> MGNDDIRQVYYEDKGISHAKAGRYSQAVMLLEQVYDADAFDVDVALHLGIAYVKTGAVDRGTELLERSLADAPDNVKVATVLGLTYVQVQKYDLAVPLLIKVAEANPINFNVR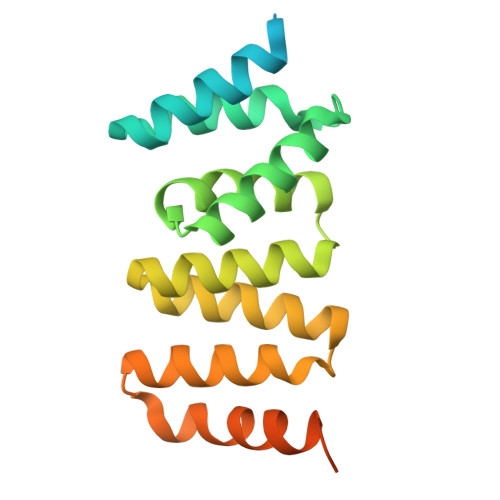FRLGVALDNLGRFDEAIDSFKIALGLRPNEGKVHRAIAFSYEQMGRHEEALPHFKKANELDEGASVELALVPRGSSAHHHHHHHHHH>[3x]MTTATAGLAVELKQSTAQAHEKAEHSTFMSDLLKGRLGVAEFTRLQEQAWLFYTALEQ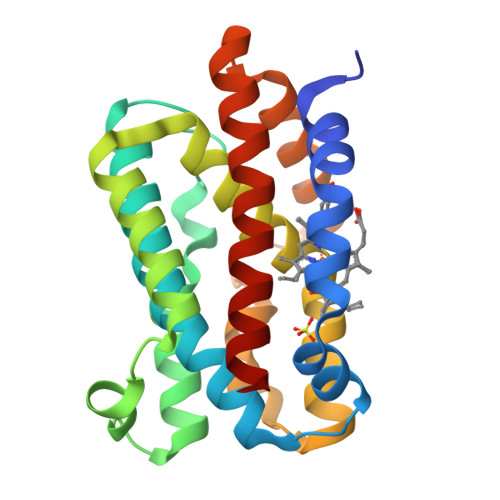AVDAVRASGFAESLLDPALNRAEVLARDLDKLNGSSEWRSRITASPAVIDYVNRLEEIRDNVDGPALVAHHYVRYLGDLSGGQVIARMMQRHYGVDPEALGFYHFEGIAKLKVYKDEYREKLNNLELSDEQREHLLKEATDAFVFNHQVFADLGKGL> MLMTVFSSAPELALLGSTFAQVDPSNLSVSDSLTYGQFNLVYNAFSFAIAAMFASALFFFSAQALVGQRYRLALLVSAIVVSIAGYHYFRIFNSWDAAYVLENGVYSLTSEKFNDAYRYVDWLLTVPLLLVETVAVLTLPAKEARPLLIKLTVASVLMIATGYPGEISDDITTRIIWGTVSTI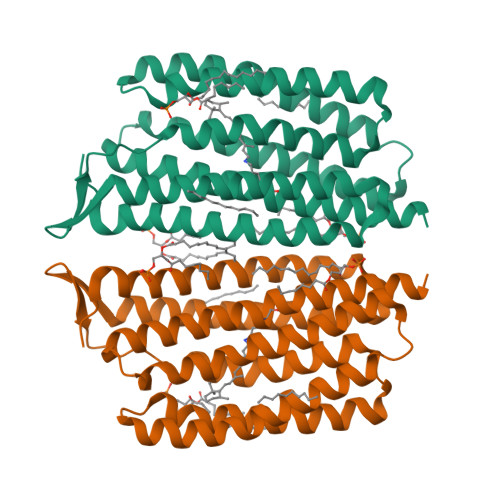PFAYILYVLWVELSRSLVRQPAAVQTLVRNMRWLLLLSWGVYPIAYLLPMLGVSGTSAAVGVQVGYTIADVLAKPVFGLLVFAIALVKTKADQESSEPHAAIGAAANKSGGSLIS> MWRVCARRAQNVAPWAGLEARWTALQEVPGTPRVTSRSGPAPARRNSVTTGYGGVRALCGWTPSSGATPRNRLLLQLLGSPGRRYYSLPPHQKVPLPSLSPTMQAGTIARWEKKEGDKINEGDLIAEVETDKATVGFESLEECYMAKILVAEGTRDVPIGAIICITVGKPEDIEAFKNYTLDSSAAPTPQAAPAPTPAATASPPTPSAQAPGSSYPPHMQVLLPALSPTMTMGTVQRWEKKVGEKLSEGDLLAEIETDKATIGFEVQEEGYLAKILVPEGTRDVPLGTPLCIIVEKEADISAFADYRPTEVTDLKPQVPPPTPPPVAAVPPTPQPLAPTPSAPCPATPAGPKGRVFVSPLAKKLAVEKGIDLTQVKGTGPDGRITKKDIDSFVPSKVAPAPAAVVPPTGPGMAPVPTGVFTDIPISNIRRVIAQRL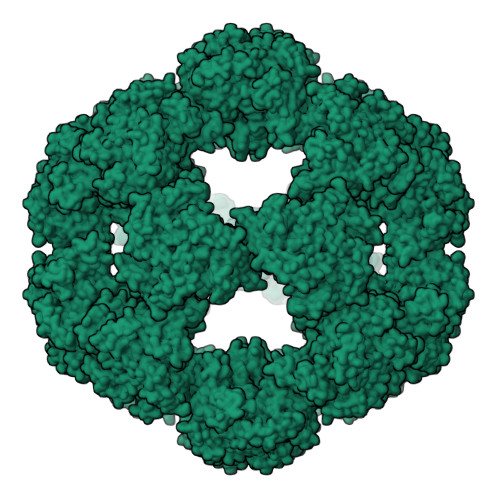MQSKQTIPHYYLSIDVNMGEVLLVRKELNKILEGRSKISVNDFIIKASALACLKVPEANSSWMDTVIRQNHVVDVSVAVSTPAGLITPIVFNAHIKGVETIANDVVSLATKAREGKLQPHEFQGGTFTISNLGMFGIKNFSAIINPPQACILAIGASEDKLVPADNEKGFDVASMMSVTLSCDHRVVDGAVGAQWLAEFRKYLEKPITMLL>SNAMARILKTAYTFDDVLLVPNKSEVLPNEVSLKTQLTKKIQLNIPLMSASMDTVTESKMAIAMAREGGIGIIHKNMTIEDQAREVDRVKRSGGLLCGASIGV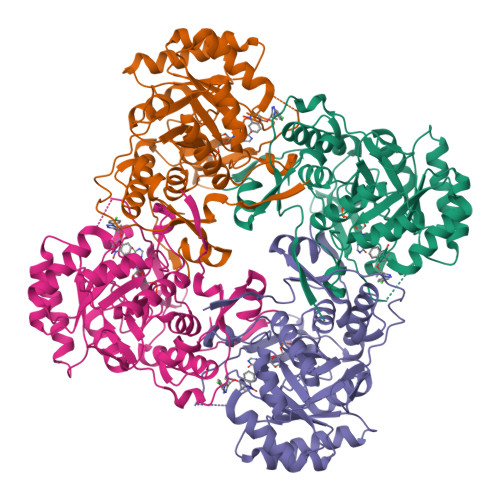TNDMMERVDAVVKAKVDVIVLDTAHGHSKGVIEGVKRIKAKYPELQVIAGNIATPEAVRDLAEAGADCVKVGIGPGSICTTRIVAGVGVPQLTAVMDCAEEGKKLGIPVIADGGLKYSGDIVKALAAGACAAMMGSIFAGCEEAPGAIEIYQGRSYKVYRGMGSLGAMAKGSSDRYFQNGTKKFVPEGVEGRIAYKGHLADTIYQLIGGIKSGMGYLGAPTLENLYENANFVVQTSAGFRESHPHDINITKEAPNYSVNQ[8x]>NADNYKNVINRTGAPQYMKDYDYDDHQRFNPFFDLG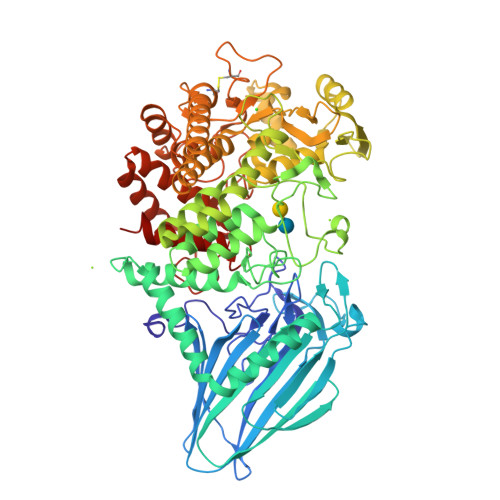AWHGHLLPDGPNTMGGFPGVALLTEEYINFMASNFDRLTVWQDGKKVDFTLEAYSIPGALVQKLTAKDVQVEMTLRFATPRTSLLETKITSNKPLDLVWDGELLEKLEAKEGKPLSDKTIAGEYPDYQRKISATRDGLKVTFGKVRATWDLLTSGESEYQVHKSLPVQTEINGNRFTSKAHINGSTTLYTTYSHLLTAQEVSKEQMQIRDILARPAFYLTASQQRWEEYLKKGLTNPDATPEQTRVAVKAIETLNGNWRSPGGAVKFNTVTPSVTGRWFSGNQTWPWNTWKQAFAMAHFNPDIAKENIRAVFSWQIQPGDSVRPQDVGFVPDLIAWNLSPERGGDGGNWNERNTKPSLAAWSVMEVYNVTQDKTWVAEMYPKLVAYHDWWLRNRDHNGNGVPEYGATRDKAHNTESGEMLFTVKKGDKEETQSGLNNYARVVEKGQYDSLEIPAQVAASWESGRDDAAVFGFIDKEQLDKYVANGGKRSDWTVKFAENRSQDGTLLGYSLLQESVDQASYMYSDNHYLAEMATILGKPEEAKRYRQLAQQLADYINTCMFDPTTQFYYDVRIEDKPLANGCAGKPIVERGKGPEGWSPLFNGAATQANADAVVKVMLDPKEFNTFVPLGTAALTNPAFGADIYWRGRVWVDQFWFGLKGMERYGYRDDALKLADTFFRHAKGLTADGPIQENYNPLTGAQQGAPNFSWSAAHLYMLYNDFFRKQ[2x]> HHHHHHATAVVRCRTRLARRVVAAVGPDGLLPAPCESRVLESALALALLTEERAEADATARLTAYLRTTLRTAPPDPFQCAVARAVLGGAGERGERVGDEGDMDAGTALDAGLDGFDHFTAGRKRLMFRTVLAALGATGFPAVPWEAYDTRPQQSWLHMEMKALKVLAAHGTGHPDVVRDEDWRALLPALEPGPAWECNNLAQLLALLALRHSPRHRPALGDVLKHVAGRLRPDGGMPFIDGMTVFTTAAAGLALSLLPAPPACVTPMADALALRRNPDGGYGFHSGVAQSDVEDTCYVLEFLRRAAPDRHRTAVAEAEGYLLALRNPDGGFPTFARGTSSEIAMTAAAASALAHDPDRREEVDEAVRYVVRHQRPDGTFERSWSRNATNAVFRAVLALTGVA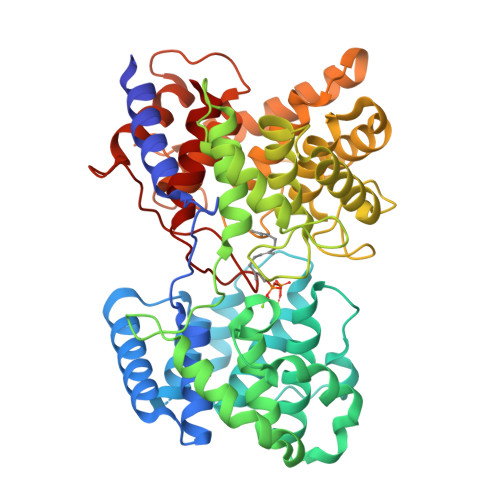AHGEERRSRARAAERALAHLAATQNGDGGWGHAEAEPSDPISTAYAVIALARGPRARPGGPLDRALAYLVERQHPDGGYRSRPDQAGPRPLLYDVPALADVFVLLALAHAT>DLEKGVVLSDLCNFLVSQTIQGWKVYWAGIEFDVTHKGMALLHRLKTNDFAPAWSMTRNLFPHLFQNPNSTIESPLWALRVILAAGIQDQLIDQSLIEPLAGALGLISDWLLTTNTNHFNMRTQRVKEQLSLKMLSLIRSNILKFINKLDALHVVNYNGLLSSIEIGTQNHTIIITRTNMGFLVELQEPDKSAMNRMKPGPAKFSLLHESTLKAFT[3x];>TQVILNCSALPCLLHLLSSPKESIRKEACWTVSNITA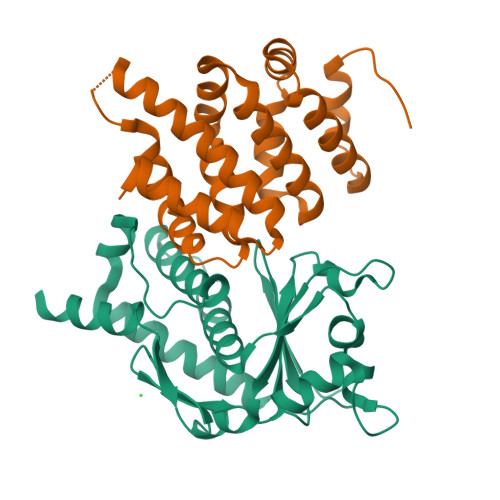GNRAQIQAVIDANIFPVLIEILQKAEFRTRKEAAWAITNATSGGTPEQIRYLVALGCIKPLCDLLTVMDSKIVQVALNGLENILRLGEQESKQNGIGINPYCALIEEAYGLDKIEFLQSHENQEIYQKAFDLIEHYFG[3x]N~2~-(3-aminobenzyl)-N~2~-[(4-fluoro-3-methylphenyl)sulfonyl]-N-hydroxy-D-alaninamide | C17 H20 F N3 O4 S | 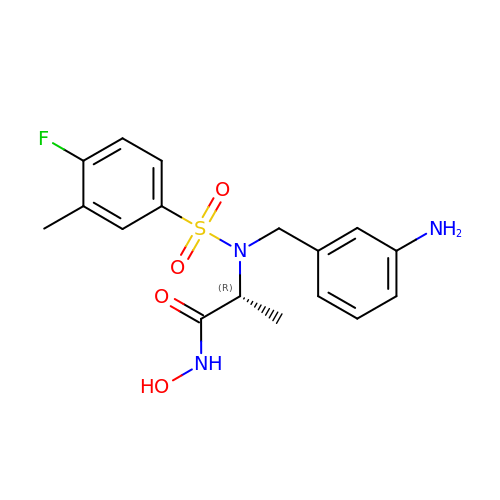OULLBGRQWIKSBM-GFCCVEGCSA-N> VGPKTGEENQVLVPNLNPTPENLEVVGDGFKITSSINLVGEEEADENAVNALREFLTANNIEINSENDPNSTTLIIGEVDDDIPELDEALNGTTAENLKEEGYALVSNDGKIAIEGKDGDGTFYGVQTFKQLVKESNIPEVNITDYPTVSARGIVEGFYGTPWTHQDRLDQIKFYGENKLNTYIYAPKDDPYHREKWREPYPESEMQRMQELINASAENKVDFVFGISPGIDIRFDGDAGEEDFNHLITKAESLYDMGVRSFAIYWDDIQDKSAAKHAQVLNRFNEEFVKAKGDVKPLITVPTEYDTGAMVSNGQPRAYTRIFAETVDPSIEVMWTGPGVVTNEIPLSDAQLISGIYNRNMAVWWNYPVTDYFKGKLALGPMHGLDKGLNQYVDFFTVNPMEHAELSKISIHTAADYSWNMDNYDYDKAWNRAIDMLYGDLAEDMKVFANHSTRMDNKTWAKSGREDAPELRAKMDELWNKLSS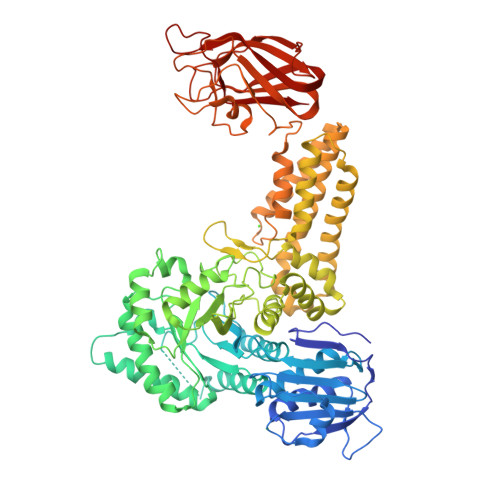KEDASALIEELYGEFARMEEACNNLKANLPEVALEECSRQLDELITLAQGDKASLDMIVAQLNEDTEAYESAKEIAQNKLNTALSSFAVISEKVAQSFIQEALSFDLTLINPRTVKITASSEETSGENAPASFASDGDMNTFWHSKWSSPAHEGPHHLTLELDNVYEINKVKYAPRQDSKNGRITGYKVSVSLDGENFTEVKTGTLEDNAAIKFIEFDSVDAKYVRLDVTDSVSDQANGRGKFATAAEVNVHG>GSMVEATAQETDRPRFSFSIAAREGKARTGTIEMKRGVIRTPAFMPVGTAATVKALKPETVRATGADIILGNTYHLMLRPGAERIAKLGGLHSFMGWDRPILTDSGGYQVMSLSSLTKQSEEGVTFKSHLDGSRHMLSPERSIEIQHLLGSDIVMAFDECTPYPATPSRAASSMERSMRWAKRSRDAFDSRKEQAENAALFGIQQGSVFENLRQQSADALAEIGFDGYAVGGLAVGEGQDEMFRVLDFSVPMLPDDKPHYLMGVGKPDDIVGAVERGIDMFDCVLPTR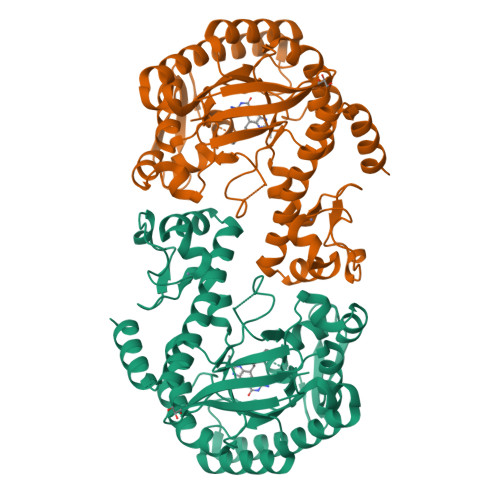SGRNGQAFTWDGPINIRNARFSEDLKPLDSECHCAVCQKWSRAYIHHLIRAGEILGAMLMTEHNIAFYQQLMQKIRDSISEGRFSQFAQDFRARYFARNS[2x]> GSSGSSGKQTGYLTIGGQRYQAEINDLENLGEMGSGTCGQVWKMRFRKTGHVIAVKQMRRSGNKEENKRILMDLD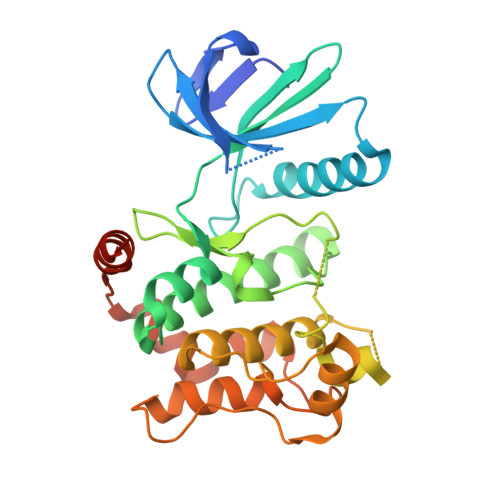VVLKSHDCPYIVQCFGTFITNTDVFIAMELMGTCAEKLKKRMQGPIPERILGKMTVAIVKALYYLKEKHGVIHRDVKPSNILLDERGQIKLCDFGISGRLVDDKAKDRSAGCAAYMAPERIDPPDPTKPDYDIRADVWSLGISLVELATGQFPYKNCKTDFEVLTKVLQEEPPLLPGHMGFSGDFQSFVKDCLTKDHRKRPKYNKLLEHSFIKRYETLEVDVASWFKDVMAKTESPRSGPSSG2-[4-(6,7-dimethoxyquinazolin-4-yl)oxy-2-methoxy-phenyl]-~{N}-(1-propan-2-ylpyrazol-4-yl)ethanamide | C25 H27 N5 O5 | 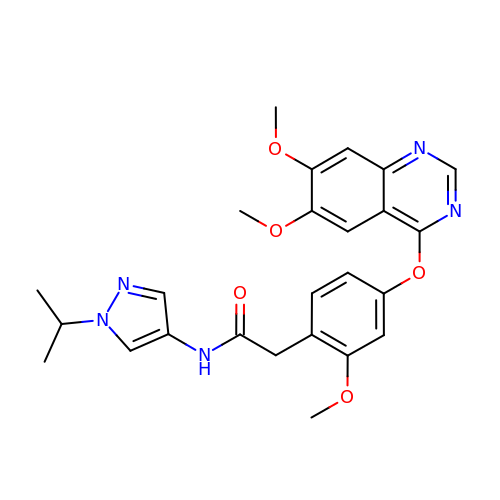INYIBEJMXPAZLV-UHFFFAOYSA-N> AYTTAQLVTAYTNANLGKAPDAATTLTLDAYATQTQTGGLSDAAALTNTLKLVNSTTAVAIQTYQFFTGVAPSAAGLDFLVDSTTNTNDLNDAYYSKFAQENRFINFSINLATGAGAGATAFAAAYTGVSYAQTVATAYDKIIGNAVATAAGVDVAAAVAFLSRQANIDYLTAFVRANTPFTAAADIDLAVKAALIGTILNAATVSGIGGYATATAAMINDLSDGALSTDNAAGVNLFTAYPSSGVSGSTLSLTTGTDTLTGTANNDTFVAGEVAGAATLTVGDTLSGGAGTDVLNWVQAAAVTALPTGVTISGIETMNVTSGAAITLNTSSGVTGLTALNTNTSGAAQTVTAGAGQNLTATTAAQAANNVAVDGGANVTVASTGVTSGTTTVGANSAASGTVSVSVANSSTTTTGAIAVTGGTAVTVAQTAGNAVNTTLTQADVTVTGNSSTTAVTVTQTAAATAGATVAGRVNGAVTITDSAAASATTAGKIATVTLGSFGAATIDSSALTTVNLSGTGTSLGIGRGALTATPTANTLTLNVNGLTTTGAITDSEAAADDGFTTINIAGSTASSTIASLVAADATTLNISGDARVTITSHTAAALTGITVTNSVGATLGAELATGLVFTGGAGADSILLGATTKAIVMGAGDDTVTVSSATLGAGGSVNGGDGTDVLVANVNGSSFSADPAFGGFETLRVAGAAAQGSHNANGFTALQLGATAGATTFTNVAVNVGLTVLAAPTGTTTVTLANATGTSDVFNLTLSSSAALAAGTVALAGVETVNIAATDTNTTAHVDTLTLQATSAKSIVVTGNAGLNLTNTGNTAVTSFDASAVTGTGSAVTFVSANTTVGEVVTIRGGAGADSLTGSATANDTIIGGAGADTLVYTGGTDTFTGGTGADIFDINAIGTSTAFVTITDAAVGDKLDLVGISTNGAIADGAFGAAVTLGAAATLAQYLDAAAAGDGSGTSVAKWFQFGGDTYVVVDSSAGATFVSGADAVIKLTGLVTLTTSAFATEVLTLA

Most bacterial and all archaeal cells are encapsulated by a paracrystalline, sheet-like, proteinaceous sheath known as a surface layer (or S-layer). In Gram-negative bacteria such as Caulobacter crescentus or Campylobacter fetus, S-layers are retained on cells by lipopolysaccharide (LPS) or endotoxin molecules present in the outer membrane (OM) (Fagan and Fairweather, 2014, Sára and Sleytr, 2000). The S-layer of C. crescentus is composed of a single, 1026-amino-acid-residue, multi-domain, S-layer protein called RsaA (Smit et al., 1992). In the case of the C. crescentus S-layer, it is remarkable how division of labor between different RsaA domains, where RsaANTD mediates cell anchoring and RsaACTD forms the lattice layer, allows this remarkable polyprotein to perform multiple tasks on the cell surface to form micron-scale, two-dimensional sheaths on membranes with variable curvature.

To obtain a more detailed view of the cellular S-layer, we used recently described subtomogram averaging algorithms (Turoňová et al., 2017) to obtain a 4.8 Å resolution structure of the S-layer lattice directly on the surface of cell stalks. The subtomogram averaging map shows large anisotropy in resolution, with the resolution highest in RsaANTD, close to the 6-fold symmetrization axis. Both the RsaANTD cryo-EM structure as well as the RsaACTD X-ray structure (Bharat et al., 2017) could be docked into the cryo-ET density unambiguously as rigid bodies. All α helices of RsaANTD are resolved in the cryo-ET map, and large side chains are resolved, which fit the density well without any further refinement. Satisfyingly, a clear density for the O-antigen of the LPS is observed in the same relative location as in the single-particle cryo-EM map of the RsaANTD:PS complex. It is worth mentioning that the RsaANTD:RsaANTD interface is almost unchanged from the interaction observed in the RsaANTD:PS spiral complex. There are very few contact sites observed between RsaANTD and RsaACTD, showing why the two domains can oligomerize independently. The two domains are connected by a short linker region, which appears as a smeared density in the cryo-ET map, suggesting some flexibility. The density for the LPS O-antigen is clearly resolved near the RsaANTD domain, and this density ends within the RsaANTD layer and does not extend outward to the RsaACTD. This indicates that upon secretion and assembly into an S-layer, RsaA proteins localize at the very tip of the O-antigen.>[2x]SMADGNEDLRADDLPGPAFESYESMELACPAERSGHVAVSDGRHMFV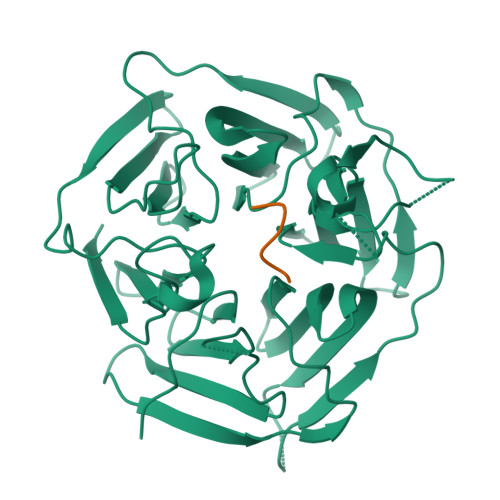WGGYKSNQVRGLYDFYLPREELWIYNMETGRWKKINTEGDVPPSMSGSCAVCVDRVLYLFGGHHSRGNTNKFYMLDSRSTDRVLQWERIDCQGIPPSSKDKLGVWVYKNKLIFFGGYGYLPEDKVLGTFEFDETSFWNSSHPRGWNDHVHILDTETFTWSQPITTGKAPSPRAAHACATVGNRGFVFGGRYRDARMNDLHYLNLDTWEWNELIPQGICPVGRSWHSLTPVSSDHLFLFGGFTTDKQPLSDAWTYCISKNEWIQFNHPYTEKPRLWHTACASDEGEVIVFGGCANNLLVHHRAAHSNEILIFSVQPK;>[2x]IGLLGG> KAMAGNFWQSSHYLQWILDKQDLLKERQKDLKFLSEEEYWKLQIFFTNVIQALGEHLKLRQQVIATATVYFKRFYARYSLKSIDPVLMAPTCVFLASKVEEFGVVSNTRLIAAATSVLKTRFSYAFPKEFPYRMNHILECEFYLLELMDCCLIVYHPYRPLLQYVQDMGQEDMLLPLAWRIVNDTYRTDLCLLYPPFMIALACLHVACVVQQKDARQWFAELSVDMEKILEIIRVILKLYEQWKNFDERKEMATILSKMPKPKPPPNSEGEQGPNGSQNSS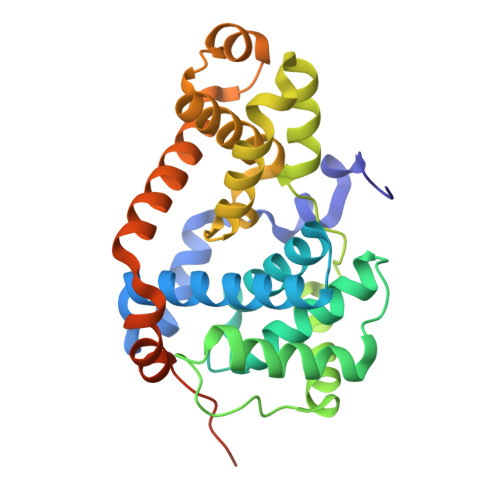YSQS> KETAAAKFERQHMDSSTSAASSSNYCNQMMKSRNLTKDRCKPVNTFVHESLADVQAVCSQKNVACKNGQTNCYQSYSTMSITDCRETGSSKYPNCAYKTTQANK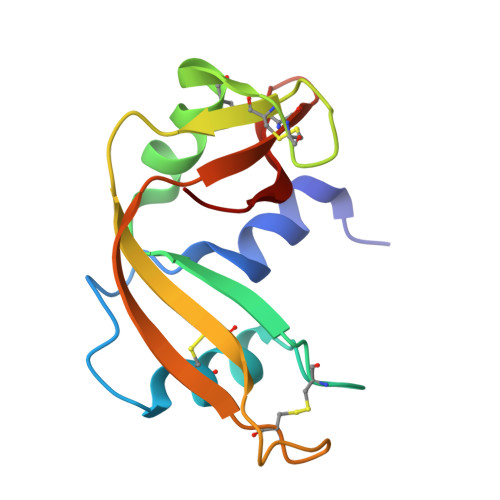HIIVACEGNPYVPVHGDASV> HHHHHHENLYFQGAADTTYVVAGTTNLTGYEWVGTPDAAPENVMTADGSVFTKTFSAVPAGKNYQLKVVANTGDEQKWIGLDGTDNNVTFDVETACDVTVTFDPATNKITVTGDGVKMVTDLEVNSITVVGNGEDNWLNGVAWGVDAEVNHMTQVSDKVYQIKYENIESADDAYQFKFAANDDWAASWGLPEQSATPIGEEFDLTFNGQNMLLNTVSAGFEEDSLVDVTITLDITNFDYSTRSGAKATVKVEPSTP

Ruminococcus bromii is a keystone species in the human gut that has the rare ability to degrade dietary resistant starch (RS). This bacterium secretes a suite of starch-active proteins that work together within larger complexes called amylosomes that allow R. bromii to bind and degrade RS. Starch adherence system protein 20 (Sas20) is one of the more abundant proteins assembled within amylosomes, but little could be predicted about its molecular features based on amino acid sequence. Here, we performed a structure–function analysis of Sas20 and determined that it features two discrete starch-binding domains separated by a flexible linker.

Furthermore, the crystal structure of a close homolog of Sas20 domain 2 revealed a unique bilobed starch-binding groove that targets the helical α1,4-linked glycan chains found in amorphous regions of amylopectin and crystalline regions of amylose. However, a single maltotriose molecule was captured between these modules with amino acids from both lobes coordinating the ligand. The aromatic ring of W509 in Sca5X25-2a interacts via van der Waals forces with the hexose ring of Glc3 at the reducing end. The O2 and O3 of Glc3 is stabilized by hydrogen bonding to the side chains of Sca5X25-2a N564 and Sca5X25-2b N684. The aromatic rings of W661 and side chain of K654 in Sca5X25-2b interact with the aglycone face and O2 of Glc2, respectively. The O6 of Glc2 is within 2.5 Å of the side chain of Sca5X25-2a E508. Glc1 interacts with W620, and its O2 and O3 coordinate with the side chain of N687. Sca5X25-2a and Sca5X25-2b overlay with an RMSD of 1.0 Å over 49 Cα atoms and demonstrate a conserved binding platform; when maltotriose is included in this overlay, the ligand displays the same polarity. The φ (O5-C1-O4’-C4′) and Ψ (C1-O4’-C4’-C5′) angles of maltotriose in our structure are φ = 107.5°, Ψ = −144.3° and φ = 90.8°, Ψ = −153.7°. The first φ/Ψ angles that is near the end of the chain is more obtuse, whereas the φ/Ψ angles cloistered within the binding cleft are similar to those found in double-helical amylose.>SGISLDNSYKMDYPEMGLCIIINNKNFHKSTGMTSRSGTDVDAANLRETFRNLKYEVRNKNDLTREEIVELMRDVSKEDHSKRSSFVCVLLSHGEEGIIFGTNGPVDLKKITNFFRGDRCRSLTGKPKLFIIQACRGTELDCGIETDSGVDDDMACHKIPVDADFLYAYSTAPGYYSWRNSKDGSWFIQSLCAML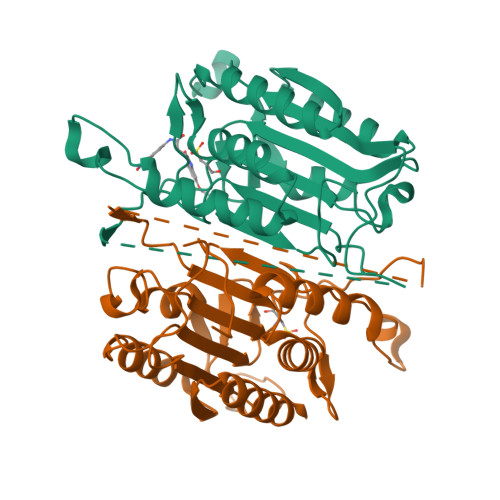KQYADKLEFMHILTRVNRKVATEFESFSFDATFHAKKQIPCIVSMLTKELYFYH[4x]> MFERFTDRARRVVVLAQEEARMLNHNYIGTEHILLGLIHEGEGVAAKSLESLGISLEGVRSQVEEIIGQGQQAPSGHIPFTPRAKKVLELSLREALQLGHNYIGTEHILLGLIREGEGVAAQVLVKLGAELTRVRQQVIQLLSGYQGKEAAEAGTGGRGGESGSPSTSLVLDQFGRNLTAAAMEGKLDPVIGREKEIERVMQVLSRRTKNNPVLIGEPGVGKTAVVEGLAQAIVHGEVPETLKDKQLYTLDLGSLVAGSRYRGDFEERLKKVLKEINTRGDIILFIDELHTLVGA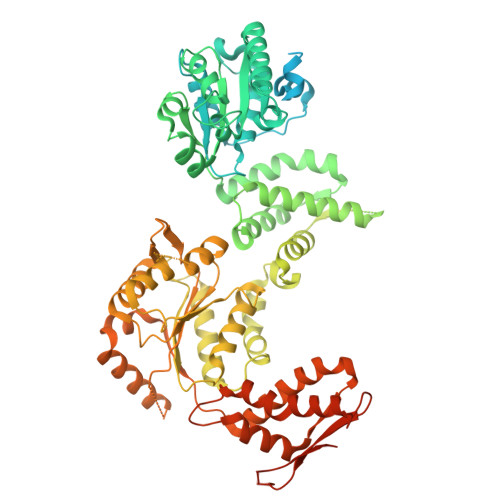GAAEGAIDAASILKPKLARGELQTIGATTLDEYRKYIEKDAALERRFQPVQVGEPTVEHTIEILKGLRDRYEAHHRVSITDAAMVAAATLADRYINDRFLPDKAIDLIDEAGARMRIRRMTAPPDLREFDEKIAEARREKESAIDAQDFEKAASLRDREKTLVAQRAEREKQWRSGDLDVVAEVDDEQIAEVLGNWTGIPVFKLTEAETTRLLRMEEELHKRIIGQEDAVKAVSKAIRRTRAGLKDPKRPSGSFIFAGPSGVGKTELSKALANFLFGDDDALIQIDMGEFHDRFTASRLFGAPPGYVGYEEGGQLTEKVRRKPFSVVLFDEIEKAHQEIYNSLLQVLEDGRLTDGQGRTVDFKNTVLIFTSNLGTSDISKPVGLGFSKGGGENDYERMKQKVNDELKKHFRPEFLNRIDDIIVFHQLTREEIIRMVDLMISRVAGQLKSKDMALVLTDAAKALLAKRGFDPVLGARPLRRTIQREIEDQLSEKILFEEVGPGQVVTVDVDNWDGEGPGEDAVFTFTGTRKPPAEPDLAKAGAHSAGGPEPAARLEHHHHHH>GMGNIYQITVEEKAEHQRTLSFE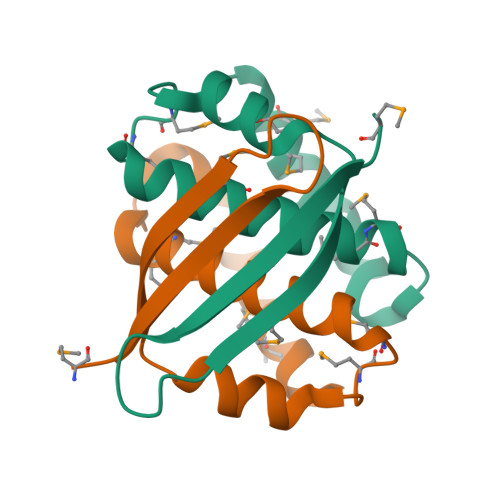FSLHDDLFKLLEKVDGKMDMTPEQTQAFMVGLKLFGEVMMQQRKHPLFKEFSAPFRAFMMNLKKQ[2x]> SWEIDPKDLTFLKELGTGQFGVVKYGKWRGQYDVAIKMIKEGSMSEDEFIEEAKVMMNLSHEKLVQLYGVCTKQRPIFIITEYMANGCLLNYLREMRHRFQTQQLLEMCKDVCEAMEYLESKQFLHRDLAARNCLVNDQGVVKVSDFGLSAYVLDDEYTSSVGSKFPVRWSPPEVLMYSKFSSKSDIWAFGVL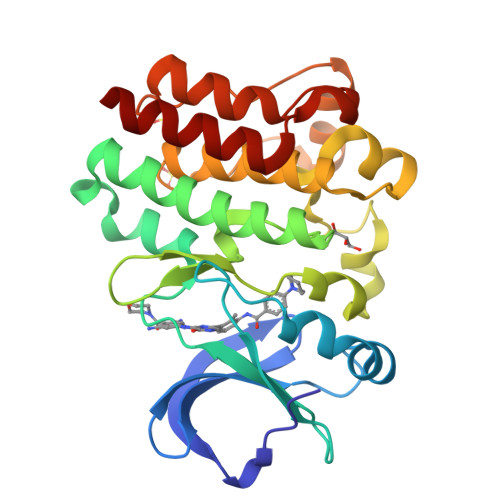MWEIYSLGKMPYERFTNSETAEHIAQGLRLYRPHLASEKVYTIMYSCWHEKADERPTFKILLSNILDVMDAN Mitochondrial calcium uptake is mediated by the mitochondrial calcium uniporter, a Ca2+-selective channel that is localized to the inner mitochondrial membrane. In humans, the uniporter functions as a holocomplex (referred to as uniplex henceforth) and consists of the pore-forming subunit MCU, an essential membrane-spanning subunit EMRE, and the gate-keeping subunits MICU1 and MICU2. The two-transmembrane (2-TM) MCU component forms a tetrameric channel pore and the single-TM EMRE becomes an integral part of the channel by forming a 1:1 stoichiometric subcomplex with MCU and renders the channel conductive. MICU1 and MICU2 are two paralogous EF-hand containing proteins that are localized to the mitochondrial intermembrane space (IMS) and function as gate-keepers by sensing the cytosolic Ca2+ concentration and, thereby, regulate MCU-EMRE channel activity.

The MICU1-MICU2 tetramer is formed by the dimerization of two MICU1-MICU2 heterodimers through a back-to-back packing between MICU2 subunits, resulting in a linear arrangement of MICU1-MICU2-MICU2-MICU1. The assembly of the MICU1-MICU2 tetramer and MCU-EMRE subcomplexes in the presence of Ca2+ is mediated by the interactions between MICU1 and EMRE. Each MICU1 subunit interacts with two EMRE subunits that are proximal to the central axis of the uniplex dimer by forming putative salt-bridge networks. Firstly, the α1 helix of MICU1 is oriented parallel to the membrane surface with its N-terminus pointing toward the C-terminal end of the transmembrane helix of EMRE. This configuration would lead to the convergence of the KKKKR poly-basic region that extends from the MICU1 α1 helix to the C-terminal poly-aspartate tail on EMRE. The second point of contact is mediated by the α11 helix of MICU1 and the poly-aspartate tail of the other EMRE subunit. The MICU1 α11 helix contains multiple basic residues whose side chains point directly toward the EMRE loop and likely form the second network of salt bridges with the poly-aspartate tail of EMRE. The binding of the MICU1-MICU2 tetramer does not block the channel pore of MCU, nor does it introduce any visible conformational change to each MCU-EMRE subcomplex, whose structure is virtually identical to that determined previously without bound MICU1 and MICU2. Thus, the uniplex structure obtained in the presence of Ca2+ represents the unblocked state in which the channel pore is poised for Ca2+ uptake.

>[8x]MAAAAGRSLLLLLSSRGGGGGGAGGCGALTAGCFPGLGVSRHRQQQHHRTVHQRIASWQNLGAVYCSTVVPSDDVTVVYQNGLPVISVRLPSRRERCQFTLKPISDSVGVFLRQLQEEDRGIDRVAIYSPDGVRVAASTGIDLLLLDDFKLVINDLTYHVRPPKRDLLSHENAATLNDVKTLVQQLYTTLCIEQHQLNKERELIERLEDLKEQLAPLEKVRIEISRKAEKRTTLVLWGGLAYMATQFGILARLTWWEYSWDIMEPVTYFITYGSAMAMYAYFVMTRQEYVYPEARDRQYLLFFHKGAKKSRFDLEKYNQLKDAIAQAEMDLKRLRDPLQVHLPLRQIGEKD;>MASGAARWLVLAPVRSGALRSGPSLRKDGDVSAAWSGSGRSLVPSRSVIVTRSGAILPKPVKMSFGLLRVFSIVIPFLYVGTLISKNFAALLEEHDIFVPEDDDDDD[8x];>[2x]MFRLNSLSALAELAVGSRWYHGGSQPIQIRRRLMMVAFLGASAVTASTGLLWKRAHAESPPCVDNLKSDIGDKGKNKDEGDVCNHEKKTADLAPHPEEKKKKRSGFRDRKVMEYENRIRAYSTPDKIFRYFATLKVISEPGEAEVFMTPEDFVRSITPNEKQPEHLGLDQYIIKRFDGKKISQEREKFADEGSIFYTLGECGLISFSDYIFLTTVLSTPQRNFEIAFKMFDLNGDGEVDMEEFEQVQSIIRSQTSMGMRHRDRPTTGNTLKSGLCSALTTYFFGADLKGKLTIKNFLEFQRKLQHDVLKLEFERHDPVDGRITERQFGGMLLAYSGVQSKKLTAMQRQLKKHFKEGKGLTFQEVENFFTFLKNINDVDTALSFYHMAGASLDKVTMQQVARTVAKVELSDHVCDVVFALFDCDGNGELSNKEFVSIMKQRLMRGLEKPKDMGFTRLMQAMWKCAQETAWDFALPKQ;>[2x]MAAAAGSCARVAAWGGKLRRGLAVSRQAVRSPGPLAAAVAGAALAGAGAAWHHSRVSVAARDGSFTVSAQKNVEHGIIYIGKPSLRKQRFMQFSSLEHEGEYYMTPRDFLFSVMFEQMERKTSVKKLTKKDIEDTLSGIQTAGCGSTFFRDLGDKGLISYTEYLFLLTILTKPHSGFHVAFKMLDTDGNEMIEKREFFKLQKIISKQDDLMTVKTNETGYQEAIVKEPEINTTLQMRFFGKRGQRKLHYKEFRRFMENLQTEIQEMEFLQFSKGLSFMRKEDFAEWLLFFTNTENKDIYWKNVREKLSAGESISLDEFKSFCHFTTHLEDFAIAMQMFSLAHRPVRLAEFKRAVKVATGQELSNNILDTVFKIFDLDGDECLSHEEFLGVLKNRMHRGLWVPQHQSIQEYWKCVKKESIKGVKEVWKQAGKGLF3-oxoheptanoic acid | C7 H12 O3 | 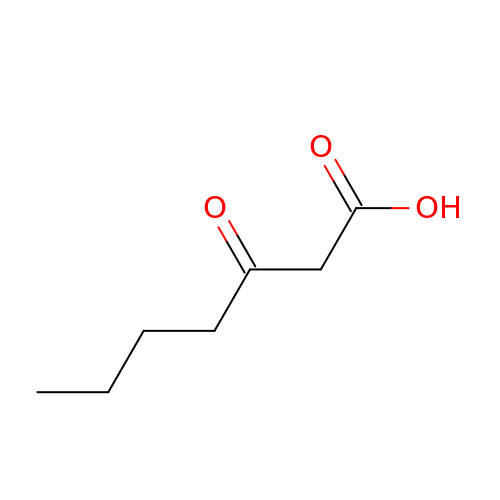PRRBQHNMYJRHFW-UHFFFAOYSA-N> SEFRGLALKYLLT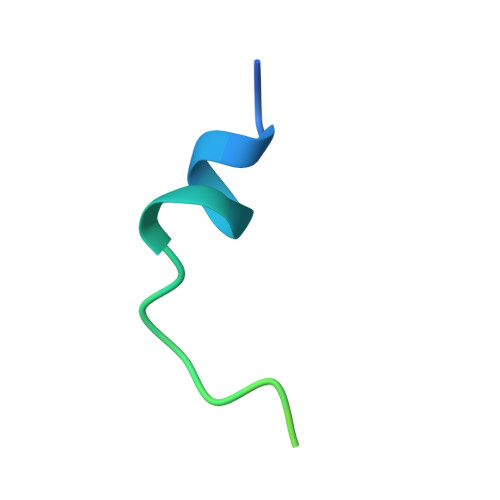PVNFFQAGYSSRRFDQQVEKYHK>[2x]GMTMFLHVVMMEFDDGIDAGF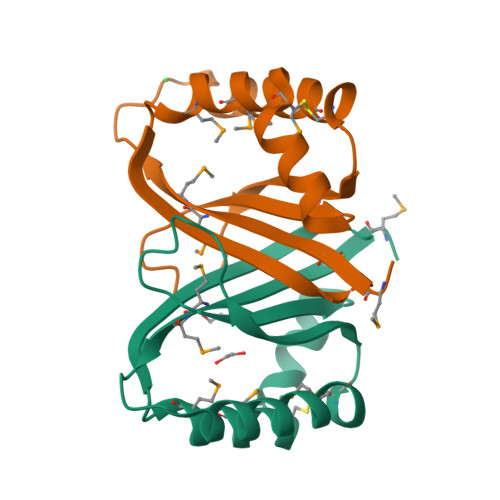FRTVDEYVARMKRECDGLLLYHFGENVAARSQGYTHATSSAFVDAAAHDAYQVCPAHVAMKAFMGPRIKRVVVYDGEVPAIG>[2x]SFTLTNKNVIFVAGLGGIGLDTSKELLKRDLKNLVILDRIENPAAIAELKAINPKVTVTFYPYDVTVPIAETTKLLKTIFAQLKTVDVLINGAGILDDHQIERTIAVNYTGLVNTTTAILDFWDKRKGGPGGIICNIGSVTGFNAIYQVPVYSGTKAAVVNFTSSLAKLAPITGVTAYTVNPGITRTTLVHKFNSWLDVEPQVAEKLLAHPTQPSLACAENFVKAIELNQNGAIWKLDLG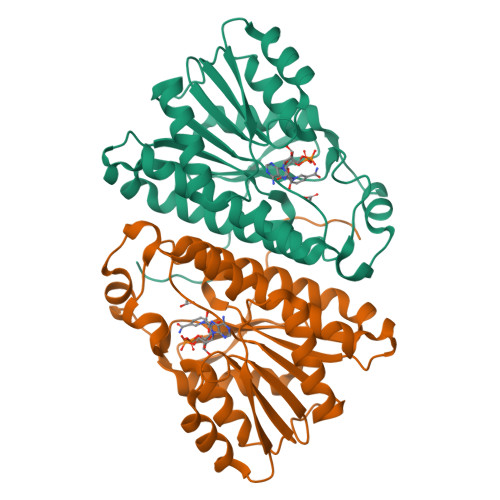TLEAIQWTKHWDSGI> QTSVSPSKVILPRGGSVLVTCSTSCDQPKLLGIETPLPKKELLLPGNNRKVYELSNVQEDSQPMCYSNCPDGQSTAKTFLTVYWTPER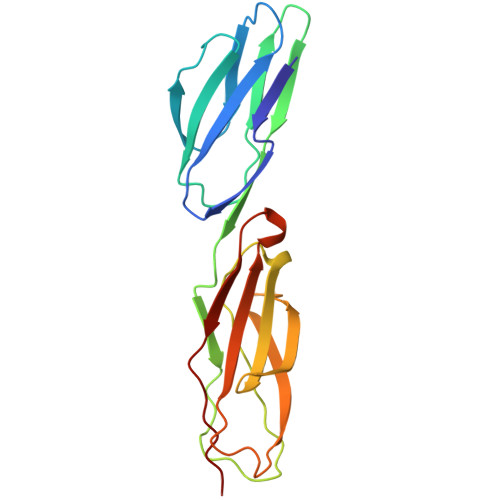VELAPLPSWQPVGKNLTLRCQVEGGAPRANLTVVLLRGEKELKREPAVGEPAEVTTTVLVRRDHHGANFSCRTELDLRPQGLELFENTSAPYQLQTF7-ethyl-10-hydroxycamptothecin | C22 H20 N2 O5 | 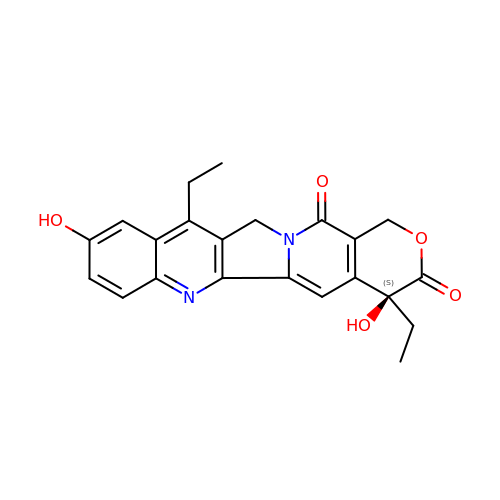FJHBVJOVLFPMQE-QFIPXVFZSA-N> GAMASGKVVKFSYMWTINNFSFCREEMGEVIKSSTFSSGANDKLKWCLRVNPKGLDEESKDYLSLYLLLVSCPKSEVRAKFKFSILNAK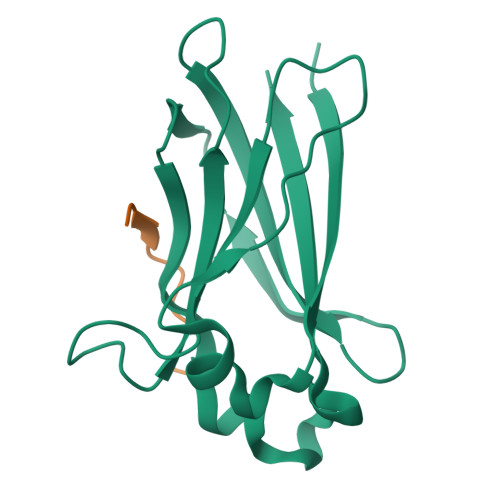GEETKAMESQRAYRFVQGKDWGFKKFIRRDFLLDEANGLLPDDKLTLFCEVSVVQD;> PEQDCAVTSGE> GSMAHSDGIFKKEQAMCLEKIQRANELMGFND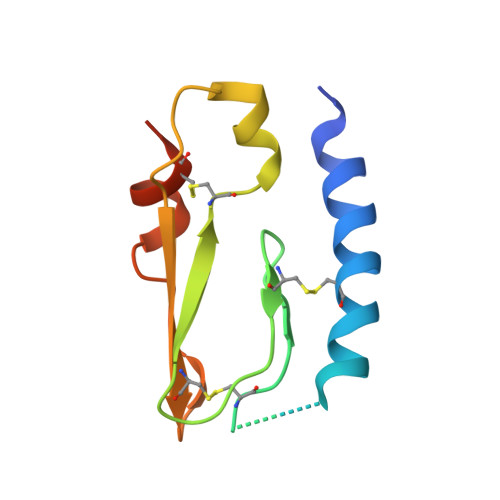SSPGCPGMWDNITCWKPAHVGEMVLVSCPELFRIFNPDQDMGVVSRNCTEDGWSEPFPHYFDACGFDEYESET> GPVATGERPTASAGHFPLTITNCGVDVTFDGPPERIILLESAPVATMRALGVLDSVVLRAGAFPPEYYDAETNAALRAIPSLGEELDSSGHLQISEEVIIAQQPDLVLGLPDGVTREGLEAVGINVLVQPTMCPGGVGATTFDDVYEQINTYGRLFDR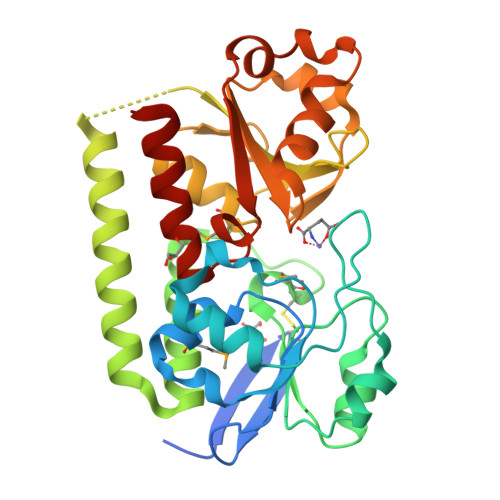QDRAAELVASLRQRVAAVEKAVEKAVGRPRRSAAVLYPTIGGGVGYAYGNESMAHPQLESAGFTNVYADVDERVFEVTLEDVLEQDPDVLVLLHVDGDPDAVKDAVVNLPGADALTAVRNDDILVQLFNFTEPPTPLSVDGLERIHETFGADS>MSMSKQVLKENMKTTYHMDGSVNGHYFTIEGEGTGNPFKGQQSLKLRVTKGGPLPFAFDILSPTFTYGNRVFTDYPEDMPDYFKQSLPEGYSWERTMMYEDGATATASARISLDKNGFVHKST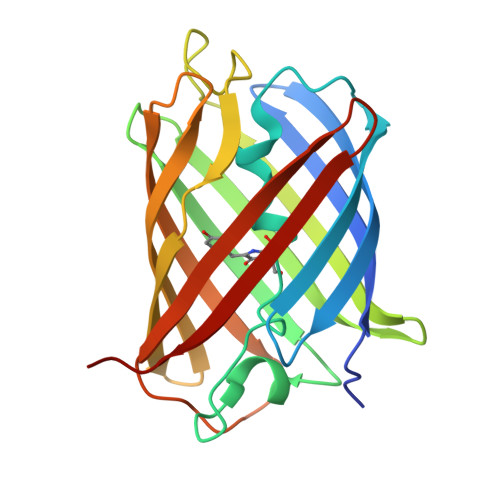FHGENFPANGPVMKKKGVNWEPSSETITPSDGILKGDVTMFLVLEGGQRLKALFQTTYKANKVVKMPPRHKIEHRLVRSEDGETIQLQEHAVAKYFTE[8x]> SAELASEAGVQQQPLELRPGEYRVLLCVDIGETRGGGHRPELLRELQRLHVTHTVRKLHVGDFVWVAQETNPRDPANPGELVLDHIVERKRLDDLCSSIIDGRFREQKFRLKRCGLERRVYLVEEHGSVHNLSLPESTLLQAVTNTQ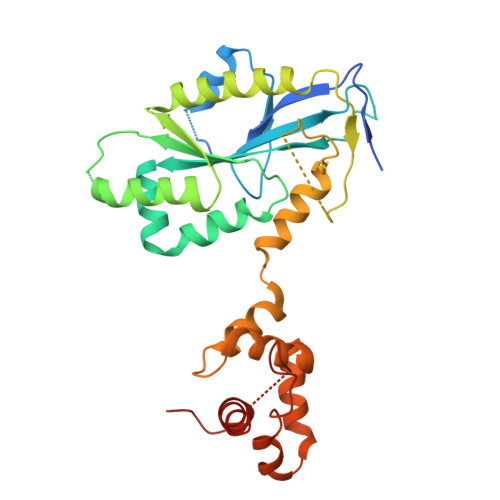VIDGFFVKRTADIKESAAYLALLTRGLQRLYQGHTLRSRPWGTPGNPESGAMTSPNPLCSLLTFSDFNAGAIKNKAQSVREVFARQLMQVRGVSGEKAAALVDRYSTPASLLAAYDACATPKEQETLLSTIKCGRLQRNLGPALSRTLSQLYCSYGPLT Immunity proteins protect the colicin producing, or “colicinogenic”, bacteria by binding and inactivating colicin nucleases with very high affinity (Kd ≈ 10− 14 M) and specificity; the discrimination in binding affinity between cognate and non-cognate nucleases by Im proteins can be up to 10 orders of magnitude. In the context of DNase bacteriocins, the HNH motif, which coordinates a single divalent metal ion within its centre, binds to the minor groove of genomic DNA causing random cleavages that overwhelm the DNA repair machinery of the cell and result in death within minutes of intoxication. The immunity protein associated with DNase colicins has an unusual mode of action; rather than binding directly to the DNase catalytic core, these proteins associate with the nuclease domain at an exosite adjacent to the enzyme active site. In this work, we have solved the first structures of the DNase domains of pyocins S2 and AP41 in complex with their cognate Im proteins, in addition to the structure of the isolated pyocin AP41 DNase domain.

We first determined the crystal structure of pyocin AP41 DNase in isolation to (i) verify that pyocin DNases adopt the HNH/ββα-Me fold and (ii) establish if Im binding causes any structural changes in the protein. Pyocin AP41 DNase domain protein crystals diffracted X-rays to 1.5 Å resolution and were found to belong to the P41212 space group. AP41 DNase domain adopts the typical mixed α/β HNH fold seen in other DNase bacteriocins. This fold is essentially identical to that of the colicin E9 and E2 DNases with RMSD values of 0.83 Å and 0.63 Å, respectively, for Cα atoms. Interestingly, AP41 DNase possesses a positively charged C-terminal extension (LKRKEK) that is not present in other nuclease domains. As with the archetypal ColE9 structure, the HNH/ββα-Me motif resembles a zinc finger where three histidine side chains coordinate a metal ion. In the AP41 DNase structure, the Ni2 + ion displays octahedral coordination geometry, which is coordinated by His738, His763 and His767; by a single water molecule from solution; and by the hydroxyl and a carbonyl oxygen from a citrate anion within the crystallisation solution. The citrate provides the equivalent coordination that is provided by the phosphate anion present in DNA bound forms of colicin DNases. We found that the AP41 DNase is most active in the presence of Ni2 + or Mg2 + ions whilst showing no detectable activity in the presence of Zn2 +. The two conserved water molecules that are seen in the pyocin AP41 DNase–Im complex are also observed in the apo AP41 DNase structure.

>DEPGVATGNGQPVTGNWLAGASQGDGVPIPSQIADQLRGKEFKSWRDFREQFWMAVSKDPSALENLSPSNRYFVSQGLAPYAVPEEHLGSKEKFEIHHVVPLESGGALYNIDNLVIVTPKRHSEIHKELKLKRKEK[2x]> MGHHHHHHMMSLMDNWKTDMESYDEGGLVANPNFEVLATFRYDPGFARQSASKKEIFETPDPRLGLRDEDIRQQIINEDYSSYLRVREVNSGGDLLENIQHPDAWKHDCKTIVCQRVEDMLQVIYERFFLLDEQYQRIRIALSYFKIDFSTSLNDLLKL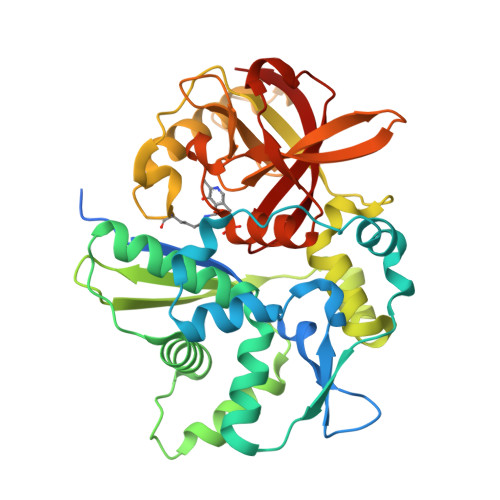LVENLINCKEGNSEYHEKIQKMINERQCYKMRVLVSKTGDIRIEAIPMPMEPILKLTTDYDSVSTYFIKTMLNGFLIDSTINWDVVVSSEPLNASAFTSFKTTSRDHYARARVRMQTAINNLRGSEPTSSVSQCEILFSNKSGLLMEGSITNVAVIQKDPNGSKKYVTPRLATGCLCGTMRHYLLRLGLIEEGDIDIGSLTVGNEVLLFNGVMGCIKGTVKTKY> LKESPSGYLRSGEGDTGCGELVWVGEPLTLRTAETITGKYGVWMRDPKPTYPYTQETTWRIDTVGTDVHQVFEYDLISQFMQGYPSKVHILPRPLESTGAVVYSGSLYFQGAESRTVIRYELNTETVKAEKEIPGAGYHGQFPYSWGGYTDIDLAVDEAGLWVIYSTDEAKGAIVLSKLNPENLELEQTWETNIRKQSVANAFIICGTLYTVSSYTSADATVNFAYDTGTGISKTLTIPFKNRYKYSSMIDYNPLEKKLFAWDNLNMVTYDIKLSKM

Inherited missense mutations in the myocilin (MYOC) gene, within its olfactomedin (OLF) domain, constitute the strongest genetic link to primary open-angle glaucoma via a toxic gain of function, and thus MYOC is an attractive precision-medicine target. Myocilin has no known function, and there is no glaucoma phenotype in Myoc knockout mice or in individuals with a homozygous N-terminal truncation mutation or hemizygous deletion of MYOC, but rare non-synonymous coding mutations lead to toxic intracellular sequestration of misfolded myocilin. However, not all mutations in MYOC cause glaucoma, and common variants are expected to be neutral polymorphisms. Among the common features associated with pathogenic myocilin misfolding, we demonstrate that a single metric, OLF thermal stability, can robustly segregate benign from early-onset disease variants.

Overall, nine variants (T256M, R296H, L303I, S313F, V329M, S331L, E352K, A427T, and V499I) were considered likely to be benign. Assessment of spent media from cells expressing each of the 16 full-length myocilin variants revealed WT-like secretion for T256M, R296H, L303I, S313F, V329M, S331L, T353I, A445V, V449I and K500R. Structural integrity was further confirmed by high-resolution crystal structures, which were solved for 11 OLF variants. No gross changes from WT OLF were detected for the structures of T293K, R296H, L303I, V329M, S331L, E352K, T353I, K398R, A445V, V449I or K500R, indicating that these mutations are accommodated within the native five-bladed β-propeller fold and do not perturb the dinuclear calcium-containing site. Interestingly, R296H has one loop comprising residues 261-266 that was difficult to model, perhaps because H296 is smaller and adopts two conformations. In addition to the five variants that we predicted initially to be benign (T293K, T353I, K398R, A445V and K500R), our study reveals seven more (T256M, R296H, L303I, V329M, S331L, E352K and V499I) that are indistinguishable from WT OLF across multiple assays. Thus, our data indicate these should also be considered benign.>[2x]MSKPSIVILGAGYGGIVAALGLQKRLNYNEADITLVNKNDYHYITTELHQPAAGTMHHDQARVGIKELIDEKKIKFVKDTVVAIDREQQKVTLQNGELHYDYLVVGLGSEPETFGIEGLREHAFSINSINSVRIIRQHIEYQFAKFAAEPERTDYLTIVVGGA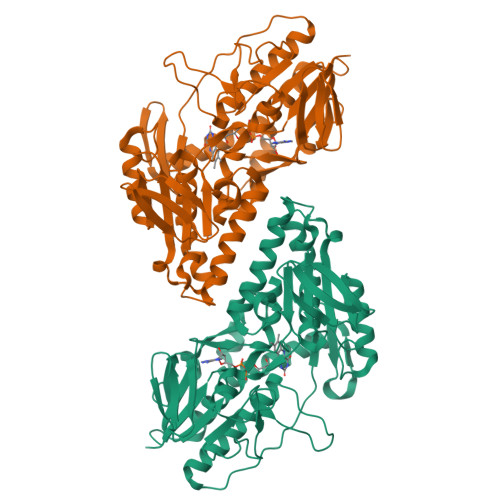EFTGIEFVGELADRMPELCAEYDVDPKLVRIINVEAAPTVLPGFDPALVNYAMDVLGGKGVEFKIGTPIKRCTPEGVVIEVDGEEEEIKAATVVWTGGVRGNSIVEKSGFETMRGRIKVDPYLRAPGHENIFIVGDCALIINEENNRPYPPTAQIAIQHGENVAANLAALIRGGSMTPFKPHIRGTVASLGRNDAIGIVGGRKVYGHAASWLKKLIDMRYLYLIGGLSLVLKKGRFHHHHHH>HPETLVTVKRIEDQLGGRLGYAELDLGSGQVLESYRGDERFPMMSTFKVLLCGAVLARVDAGQEQLDRRITYTKADLVTYSPVTEKHVGDGMTVAELCEAAITMSDNTAANLLLTTIGGPEALTAFLRSIGDTTTRLDRWETELNEALPGDPRDTTTPEAMAATLRKLLLGDVLTPASRQQLIDWMEADKVAGPLIRSALPAGWRIADKTGAGERGSRGIIALLGPPGKAPRIVVIYLTGSKADMAERNKAIAEIGAALIKHW[2x]

The TEM-1 β-lactamase model system has been extensively used to study protein evolution. β-lactamases are a class of enzymes that are produced by bacteria in order to provide resistance to bactericidal β-lactam antibiotics through hydrolysis of their core β-lactam ring. We apply EVcouplings to computationally design variants of the model protein TEM-1 β-lactamase. To examine the structural effects of these mutations, we obtained X-ray crystal structures of designs 80.a, 80.b, and 70.a. Aligning these structures in 3D to a published WT TEM-1 structure (PDB: 1XPB34) revealed that all three have nearly identical Cα backbones to WT TEM-1 (0.26–0.61 Å RMSD over all Cα atoms).

We also searched for local structural changes by examining differences in all pairwise distances between residues, which showed small changes in a one looped region for all three structures (positions 255–257) and in a second loop of 70.a (positions 53–55). Both 80.a and 80.b have 55 amino acid substitutions relative to WT TEM-1, of which 80.a has 15 mutations in the core of the structure and 80.b has 19 in the core. In particular, the 80.a and 70.a designs had between 4-fold and 32-fold increased MIC of four tested antibiotics as well as 24 °C and 6 °C increased Tm, respectively. The 80.a and 80.b designs also had a 4-fold increased MIC of aztreonam, as well as a 16-fold increased MIC of ceftazidime. The two designs that were optimized solely for predicted fitness (i.e., distance unconstrained) both conferred resistance to ampicillin, with the greedy optimized sequence (opt.a) having a MIC equal to WT TEM-1, and the parallel tempering optimized sequence (opt.b) had a large decrease in MIC (roughly 100X less). In summary, nearly all of the designs were able to confer resistance to ampicillin including a design with 84 mutations relative to its closest natural homolog (70.a) and two designs with over 50 mutations (80.a and 80.b). To investigate the structural basis for the increased Tm (80.a had a 24 °C increase relative to WT TEM-1, 80.b had a 18 °C increase, and 70.a had a 6.3 °C increase), we tallied the total number of hydrogen bonds and the number of atom pairs in contact (1.7–4 Å) in each structure. However, we did observe literature-reported globally stabilizing mutations such as M182T in every one of the designed sequences, which has been shown to confer a 7.5 °C increase in Tm as a single substitution. The 70.a, 80.a and 80.b designs also showed increased resistance to aztreonam (80.a and 80.b had a 4-fold increased MIC, and 70.a had a 32-fold increase MIC, see broth microdilution assay in Figs. 4, 5). There are five shared mutations near the active site that are in three designs (M69A, E104T, P167T, E168A, E240G) that may contribute to this increased resistance.Histones are conserved DNA-packaging proteins found across all domains of life. Here, we describe HLp from Leptospira perolatii and show by crystallographic and biophysical analyses that, unlike HBb, it forms stable tetramers and binds DNA nonspecifically, wrapping ~60 bp of DNA around its core. The HLp monomer exhibits the characteristic histone fold, comprising three α-helices (α1, α2, and α3) connected by two loops (l1 and l2). Molecular dynamics simulations, DNA-binding assays, and heterologous expression in Escherichia coli, where HLp reorganizes the nucleoid, support a role in bacterial chromatin organization.

The best data set was processed to a resolution of 1.30 Å, and the structure was solved by molecular replacement using a dimeric AF model as the search template. The entire chain, except for the first seven residues, was well resolved in the electron density map. The asymmetric unit contained an HLp dimer, which assembles into a homotetramer by crystallographic symmetry. Within the dimer, the monomers are arranged in a head-to-tail orientation, with the interface formed primarily by the antiparallel crossing of the α2 helices at an angle of ~40°. It is stabilized by hydrophobic interactions involving residues V16 and I20 (α1 helix), a leucine-rich stretch in the α2 helix (L35, L39, L42, and L47), and F63 (α3 helix), along with polar contacts between loop regions. HLp tetramers assemble through two equivalent, spatially separated interfaces formed by the C-terminal α2 helices, l2 loops, and the α3 helices of opposing dimers. Dimer-dimer contacts are stabilized by a branched hydrogen-bonding network involving R49, S52, and N53 of one monomer and F63, T61, and R55 of the opposing monomer. HLp also harbors a conserved RD-clamp—an intramolecular salt bridge between R55 and D62—that stabilizes loop l2, a feature shared with both HMfB and HBb. Nevertheless, electrostatic surface potential analysis of the HLp tetramer reveals a continuous band of positive charge encircling the structure, consistent with a DNA-wrapping mode of interaction. The central α2 helix is one turn shorter than in the archaeal histone HMfB, while the C-terminal α3 helix is truncated and forms a single helical turn composed of the final four residues—similar to what is observed in the bacterial dimeric histone HBb from B. bacteriovorus.

>GSMAQNAEKDTLIVASKVKAYIKSKGFMTSGDAVDGLNEKLYALIDDALKRTESNKRTTVRPTDF[2x]3,6-O-dimethyl-D-glucose | C8 H16 O6 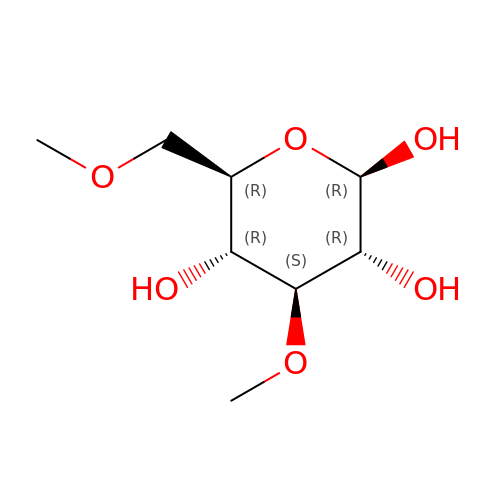| HXTJYTSBXOATMS-UIAUGNHASA-N> MAVKVEYDLKRLRNIGIAAHIDAGKTTTTERILYYTGRIHKIGEVHEGAATMDFMEQERERGITITAAVTTCFWKDHRINIIDTPGHVDFTIEVERSMRVLDGAIVVFDSSQGVEPQSETVWRQAEKYKVPRIAFANKMDKTGADLWLVIRTMQERLGARPVVMQLPIGREDTFSGIIDVLRMKAYTYGNDLGTDIREIPIPEEYLDQAREYHEKLVEVAADFDENIMLKYLEGEEPTEEELVAAIRKGTIDLKITPVFLGSALKNKGVQLLLDAVVDYLPSPLDIPPIKGTTPEGEVVEIHPDPNGPLAALAFKIMADPYVGRLTFIRVYSGTLTSGSYVYNTTKGRKER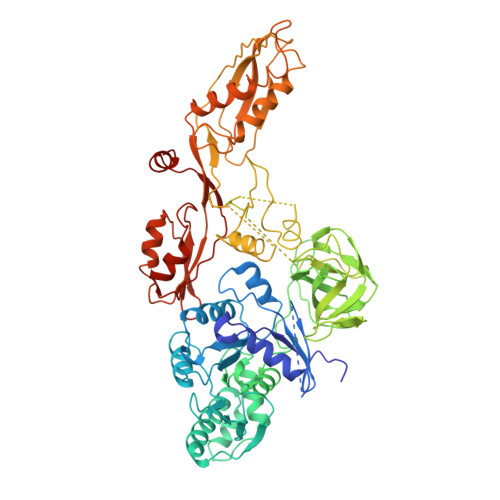VARLLRMHANHREEVEELKAGDLGAVVGLKETITGDTLVGEDAPRVILESIEVPEPVIDVAIEPKTKADQEKLSQALARLAEEDPTFRVSTHPETGQTIISGMGELHLEIIVDRLKREFKVDANVGKPQVAYRETITKPVDVEGKFIRQTGGRGQYGHVKIKVEPLPRGSGFEFVNAIVGGVIPKEYIPAVQKGIEEAMQSGPLIGFPVVDIKVTLYDGSYHEVDSSEMAFKIAGSMAIKEAVQKGDPVILEPIMRVEVTTPEEYMGDVIGDLNARRGQILGMEPRGNAQVIRAFVPLAEMFGYATDLRSKTQGRGSFVMFFDHYQEVPKQVQEKLIKGQ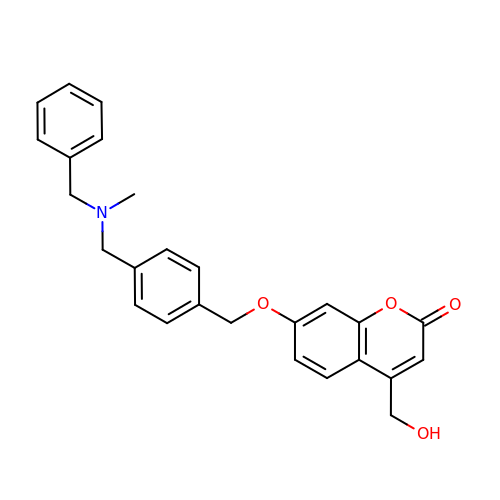4-(hydroxymethyl)-7-[[4-[[methyl-(phenylmethyl)amino]methyl]phenyl]methoxy]chromen-2-one | C26 H25 N O4 | RTJRBYKZQSYWCM-UHFFFAOYSA-N> GPMDETGK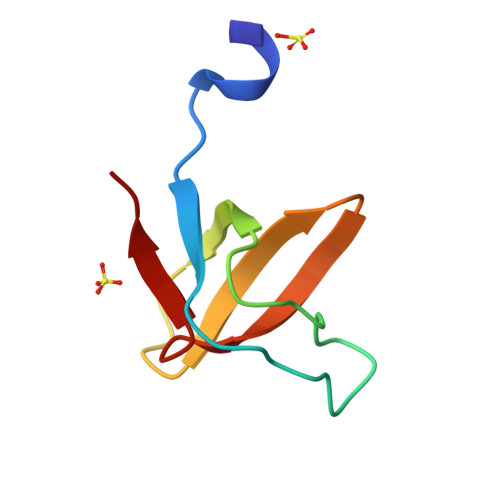ELLLVLYDYQEKSPREVTVKKGDILTLLNSTNKDWWKVEFNDRQGFVPAAYLKKLD The titular member of this family, phosphatidylcholine transfer protein (PC-TP a.k.a STARD2), specifically binds and transfers phosphatidylcholine (PC) generated in the endoplasmic reticulum throughout the cell to modulate plasma membrane, lipid, and thermal homeostasis. Steroidogenic acute regulatory lipid transport (START/STARd) domain-containing proteins bind and transport glycerophospholipids, ceramides, and sterols. The STARD2 subfamily, containing STARD2, 7, and 10, bind glycerophospholipids species. We demonstrate that PC-TP interacts directly with PPARδ to suppress its transcriptional activity, using a combination of cellular assays and binding assays with purified proteins.

C 2.18 Å structure of PC-TP in complex with PC 36:4 (PAPC) used to design proposed mutations to alter PC-TP PC binding. PC-TP adopted the expected STARd fold consisting of nine antiparallel beta sheets with four alpha helices. Our structure revealed clear electron density to guide the modeling of the bound ligand. The PC (16:0/20:4) phosphate group is coordinated by Tyr72, Arg78, and Gln157. Whereas the quaternary ammonium on the choline head group is stabilized by an aromatic cage consisting of Trp101, Tyr114, Tyr116, and Tyr155. E This structure suggests PC-TP selectivity for PCs is driven via aromatic residues that form a cage surrounding the choline head group (shown in melon) and residues that coordinate the phosphate backbone (shown in baby blue) (cutoff of 3.5 Å). Using this structure, we designed mutations to reduce phospholipid binding (R78E, R78A, and Y114R). Mutating Arg78 to glutamic acid (R78E) introduces a charge repulsion with the lipid phosphate group that would displace PL binding, where mutation of Arg78 to alanine (R78A) may have a more subtle effect by neutralizing the charge rather than introducing charge repulsion. We also mutated Y114 to an arginine to disfavor PC binding through charge repulsion. Protein complementation assays in Huh7 cells, Y114R, R78E, and R120H all decrease the interaction between PC-TP and PPARδ by ~45% relative to wild-type PC-TP.

> MELAAGSFSEEQFWEACAELQQPALAGADWQLLVETSGISIYRLLDKKTGLYEYKVFGVLEDCSPTLLADIYMDSDYRKQWDQYVKELYEQECNGETVVYWEVKYPFPMSNRDYVYLRQRRDLDMEGRKIHVILARSTSMPQLGERSGVIRVKQYKQSLAIESDGKKGSKVFMYYFDNPGGQIPSWLINWAAKNGVPNFLKDMARACQNYLKKT> GADDVVDSSKSFVMENFSSYHGTKPGYVDSIQKGIQKPKSGTQGNYDDDWKEFYSTDNKYDAAGYSVDNENPLSGKAGGVVKVTYPGLTKVLALKVDNAETIKKELGLSLTEPLMEQVGTEEFIKRFGDGASRVVLSLPFAEGSSSVEYINNWEQAKALSVELEINFETRG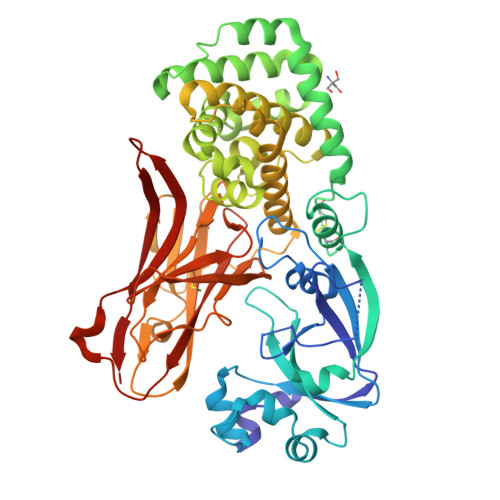KRGQDAMYEYMAQACAGNRVRRSVGSSLSCINLDWDVIRDKTKTKIESLKEHGPIKNKMSESPNKTVSEEKAKQYLEEFHQTALEHPELSELKTVTGTNPVFAGANYAAWAVNVAQVIDSETADNLEKTTAALSILPGIGSVMGIADGAVHHNTEEIVAQSIALSSLMVAQAIPLVGELVDIGFAAYNFVESIINLFQVVHNSYNRPAYSPGHKTQPFLHDGYAVSWNTVEDSIIRTGFQGESGHDIKITAENTPLPIAGVLLPTIPGKLDVNKSKTHISVNGRKIRMRCRAIDGDVTFCRPKSPVYVGNGVHANLHVAFHRSSSEKIHSNEISSDSIGVLGYQKTVDHTKVNSKLSLFFEIKS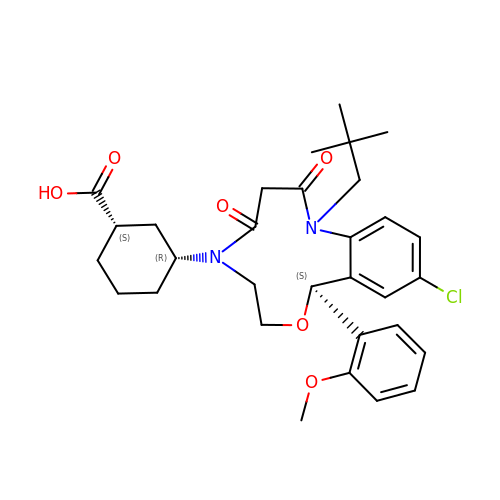(1~{S},3~{R})-3-[(10~{S})-13-chloranyl-2-(2,2-dimethylpropyl)-10-(2-methoxyphenyl)-3,5-bis(oxidanylidene)-9-oxa-2,6-diazabicyclo[9.4.0]pentadeca-1(15),11,13-trien-6-yl]cyclohexane-1-carboxylic acid | C31 H39 Cl N2 O6 | CJHFRTFWDPUFCC-APLXEUBXSA-N The pathway sensitivity is adjusted by the coordinated action of the CheR methyltransferase and the CheB methylesterase that catalyze methylation and demethylation, respectively, of several glutamate residues at the chemoreceptor-signaling domain. CheB is composed of a phosphoryl group-accepting receiver domain (REC) and a methylesterase domain, and it was shown that REC domain phosphorylation stimulates the catalytic activity of CheB. However, Tar possesses a C-terminal pentapeptide that is tethered to the C-terminal end of the chemoreceptor signaling domain via an unstructured linker. This pentapeptide, NWETF, represents an additional binding site for CheR and CheB. To this end, we chose P. atrosepticum SCRI1043 as a model that has a single CheB and 19 chemoreceptors with a pentapeptide.

To address this issue, we crystallized CheB_Pec and solved its three-dimensional structure at a resolution of 2.3 Å. The enzyme is composed of an N-terminal REC domain and a C-terminal methylesterase domain that are connected by a linker of approximately 25 amino acids. The asymmetric unit contains five CheB_Pec chains that can be closely superimposed onto each other, resulting in Cα root mean square deviation (RMSD) values of 0.23 to 0.61 Å. In each CheB_Pec chain, there was a gap due to a lacking electron density that, depending on the chain, extended from amino acids 137 to 144–150. Lacking electron density is generally attributed to the corresponding protein segment being disordered. The gap was flanked by a segment with high B-factor values, indicative of significant protein flexibility in this region. However, microcalorimetric titrations conducted with all nine pentapeptides and at different analysis temperatures did not show any sign of binding. The answer to this question may be related to studies that have identified the pentapeptide-binding site at E. coli CheB. This binding site was found to comprise amino acids 130 to 140 (colored in red in Figure 7A,B) and is located on the C-terminal extension of the REC domain and N-terminal part of the linker. The inspection of the sequence alignment of CheB from E. coli and P. atrosepticum SCRI1043 revealed a high degree of sequence divergence in the pentapeptide-binding area. Importantly, a large part of the E. coli CheB pentapeptide-binding site overlaps with the gap observed in the CheB_Pec structure (shaded in grey in Figure 7B). We therefore hypothesize that the structural disorder of CheB_Pec in the region homologous to the pentapeptide-binding site in E. coli may be related to the failure to bind pentapeptides.

>GSHMASMSKIRVLCVDDSALMRQIMTEIINSHPDMEVVATAPDPLVARDLIKKFNPQVLTLDVEMPRMDGLDFLEKLMRLRPMPVVMVSSLTGKGSEITLRALELGAIDFVTKPQLGIREGMLAYSELIAEKIRMAAKARLPQRSTTAEPTKIIQHMPLLSSEKLIAIGASTGGTEAIRHVLQPLPPTSPALLITQHMPPGFTKSFAERLNKLCQITVKEAEDGERVLPGHAYIAPGARHLELARSGANYQVRLNDGPPVNRHRPSVDVLFRSVAQYAGRNAVGVILTGMGNDGAAGMLELHQAGAYTLAQNEASCVVFGMPREAIAMGGVDEVVDLHQVSQRMLAQISAGQALRI[5x]>GMSIPANNSPVRLALIGAGRWGKNYIRTIAGLPGAALVRLASSNPDNLALVPPGCVIESDWRSVVSAPEVEAVIIATPPATHAEITLAAIASGKAVLVEKPLTLDLAEAEAVAAAAKATGVMVWVEHTQLFNPAWEALKADLTSIGPILAVRSEAGNHGPYRPGGVPMLWDWGAHDVSMVLDLMGRDPDSTSASWAARGEKDGGEAGDVTLTLAFSTVEAHIRLCNTMDKCRRLAVFGEAGTLVMDDRATDKLTLHPPQPDGNWPVGQGHALTVTDEMPLTRAVRL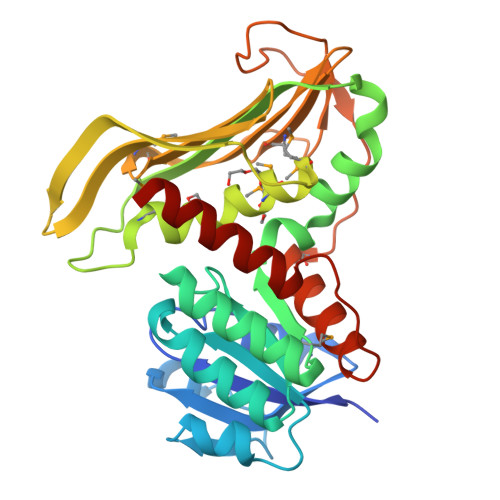FAGAVRQPEPGPSPLELGLRVVRVLGACS[2x]> MSSNEEVFTQINATANVVDNKKRLLFVQDSSALVLGLVAGFLQIESVHGFIWFLILYNLINVIYIVWICQLQPGKFYQSPLQDIFFESFFR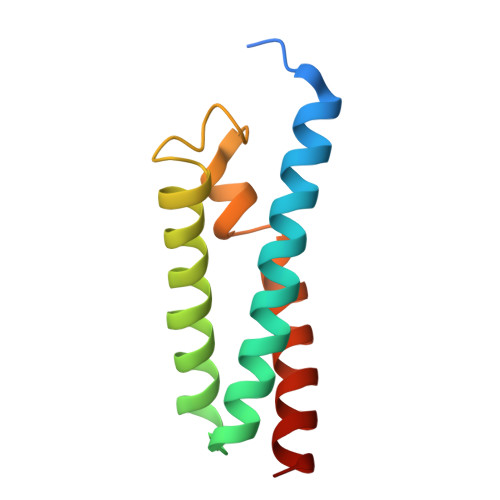EITGFVMAWTFGYALIG>MARIRHVQGDITEFQGDAIVNAANNYLKLGAGVAGAILRKGGPSIQEECDRIGKIRVGEAAVTGAGNLPVRYVIHAAVLGDEPASLETVRKATKSALEKAVELGLKTVAFTGVGAWVGGLPAEAVYRVMLEEIKKAPDTL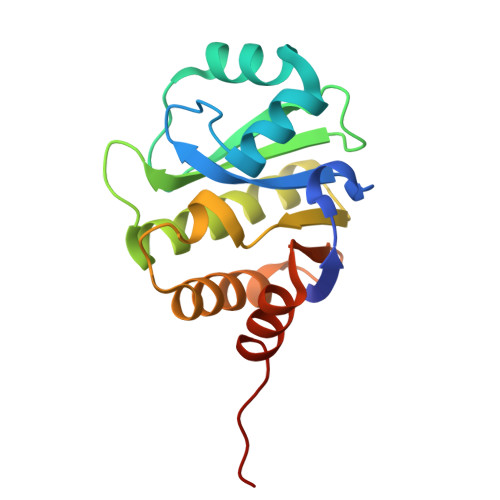EVTGVHGTEKSAEAFRRAGLEHHHHHH[4x]>MGMKLLVVSWGDFERAKETKYRFGGETSVGPSTLPILQKVIKPDWTVIVLSDTIGKDFSSVETLREDVRNRVMDFLDRIGAGREVDVIIAPGIGEFTHGSFRGSAMDAYYYVLHALSEIIPTKGDLEVHFDSTHGLNYVTLLTYRALKDLLGIAAVMNTVTFYAYNSDPFVPKITKELNINTIETTMVKPTPLSEPLPGFDEYLCPYSMERAEFVRLKGSLNTLKNLRKEKKKLEAWIGSLLFGLPLLFLEEFPDIGRLESYIEELAETWGGAIAVNAEEKAVTRRLAFGSGFGTL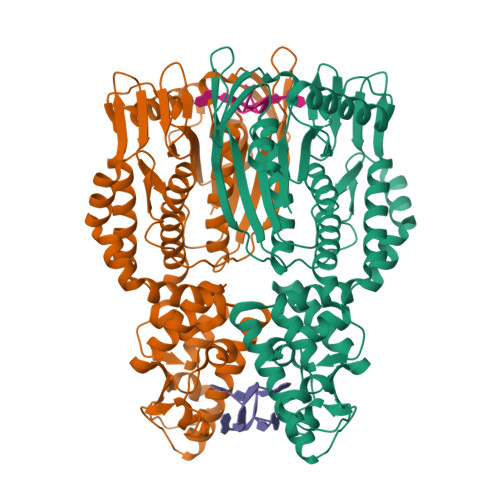VKLLFQARITRGLLVEEPYSIEKLYSVSDRLFRGSTLQRVRVALGKIEDKAIKYARKGAFPRDIPLRDFLGFDAANREVSPRNVLAHAGLEANVVEVSMEAWEPKRPEEEAGRHTHLKYTPVGLKKVEDIVSRALKESHHHHHH[2x]>[2x]PK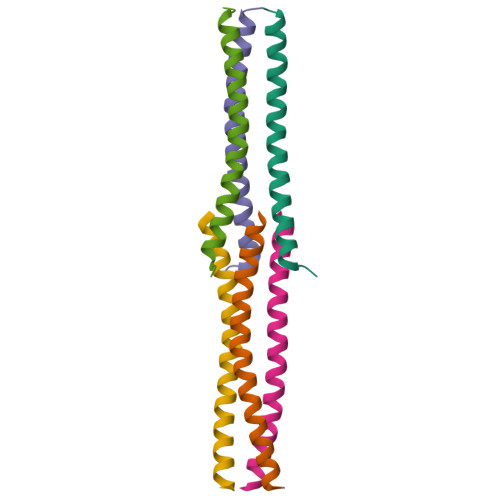TVQDLTSVVQTLLQQMQDKFQTISDQIIGRIDDMSSRIDDLEKNIA>[4x]GASGSMIVFDSDGDFLRNGGTYMLSPPNGGGGILAAAIKQGSDRDCSLGVIQHES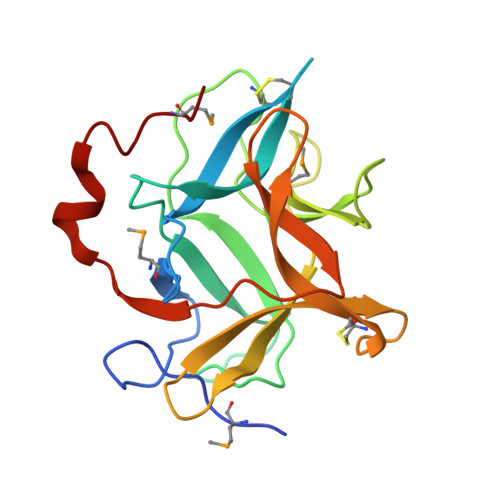YTGWPVTISALVRPTFISTSFQLLLSFAYIPPNVCTKNSDWIIKSSNDFEGTVMLGDDKNPVGSLFFIKSYDSSKNYYKLVVCGGRGDEHCRNIGVDKDENGYKRLVVTEGEPLVLQFDKVNKGNFAFESNLSMVV>[4x]AEEFPVPNGFESAYREVDGVKLHYVKGGQGPLVMLVHGFGQTWYEWHQLMPELAKRFTVIAPDLPGLGQSEPPKTGYSGEQVAVYLHKLARQFSPDRPFDLVAHDIGIWNTYPMVVKNQADIARLVYMEAPIPDARIYRFPAFTAQGESLVWHFSFFAADDRLAETLIAGKERFFLEHFIKSHA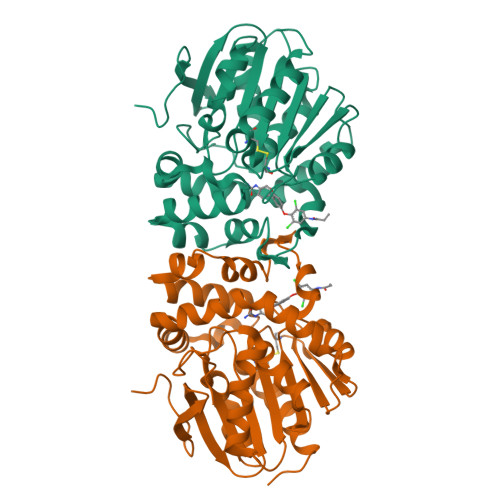SNTEVFSERLLDLYARSYAKPHSLNASFEYYRALNESVRQNAELAKTRLQMPTMTLAGGGHGGMGTFQLEQMKAYAEDVEGHVLPGCGHWLPEECAAPMNRLVIDFLSRGRHHHHHH> MRVNNGLTPQELEAYGISDVHDIVYNPSYDLLYQEELDPSLTGYERGVLTNLGAVA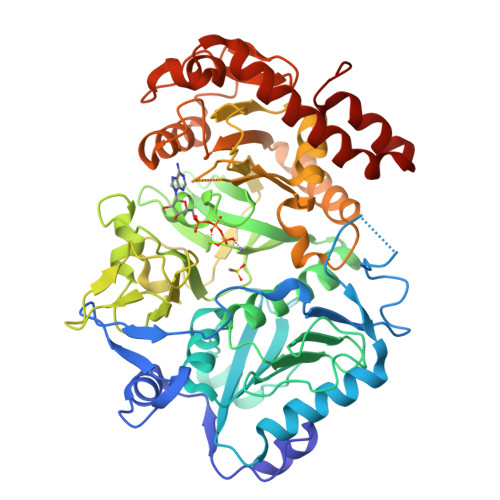VDTGIFTGRSPKDKYIVRDDTTRDTFWWADKGKGKNDNKPLSPETWQHLKGLVTRQLSGKRLFVVDAFCGANPDTRLSVRFITEVAWQAHFVKNMFIRPSDEELAGFKPDFIVMNGAKCTNPQWKEQGLNSENFVAFNLTERMQLIGGTWYGSEMKKGMFSMMNYLLPLKGIASMHCSANVGEKGDVAVFFGLSGTGKTTLSTDPKRRLIGDDEHGWDDDGVFNFEGGCYAKTIKLSKEAEPEIYNAIRRDALLENVTVREDGTIDFDDGSKTENTRVSYPIYHIDNIVKPVSKAGHATKVIFLTADAFGVLPPVSRLTADQTQYHFLSGFTAKLAGTERGITEPTPTFSACFGAAFLSLHPTQYAEVLVKRMQAAGAQAYLVNTGWNGTGKRISIKDTRAIIDAILNGSLDNAETFTLPMFNLAIPTELPGVDTKILDPRNTYASPEQWQEKAETLAKLFIDNFDKYTDTPAGAALVAAGPKLHHHHHH3-[(3~{S},4~{R})-4-azanyl-4-carboxy-pyrrolidin-3-yl]propyl-tris(oxidanyl)boranuide | 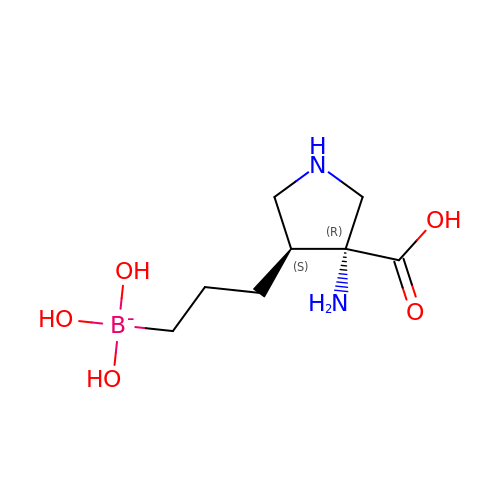C8 H18 B N2 O5 | JNNZQSJBRFVUJB-XPUUQOCRSA-N>[2x]MATQRAHRAETPAHPNRLWIWEKHVYLDEFRRSWLPVVIKSNEKFQVILR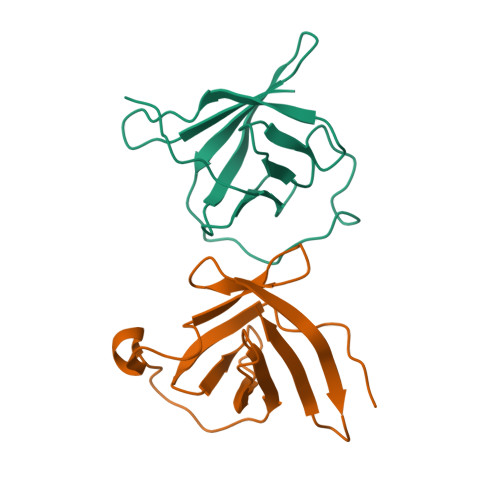QEDVTLGEAMSPSQLVPYELPLMWQLYPKDRYRSADSMYWQILYHIKFRDVEDMLLELIDSESNDE>MNPAAEAEFNILLATDSYKVTHYKQYPPNTSKVYSYFECREKKTENSKLRKVKYEETVFYGLQYILNKYLKGKVVTKEKIQEAKDVYKEHFQDDVFNEKGWNYILEKYDGHLPIEIKAVPEGFVIPRGNVLFTVENTDPECYWLTNWIETILVQSWYPITVATNSREQKKILAKYLLETSGNLDGLEYKLHDFGYRGVSSQETAGIGASAHLVNFKGTDTVAGLALIKKYYGTKDPVPGYSVPAAEHSTITAWGKDHEKDAFEHIVTQFSSVPVSVVSDSYDIYNACEKIWGEDLRHLIVSRSTQAPLIIRPDSGNPLDTVLKVLEILGKKFPVTENSKGYKLLPPYLRVIQG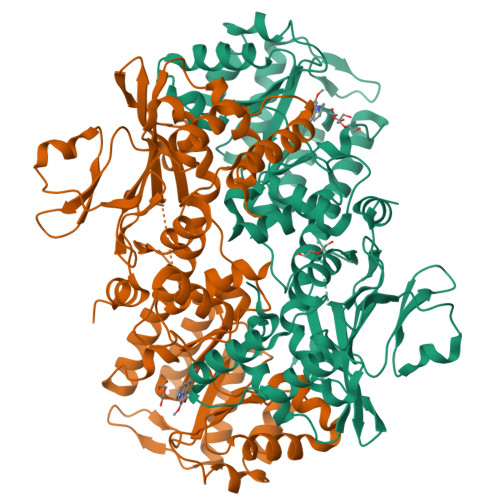DGVDINTLQEIVEGMKQKMWSIENIAFGSGGGLLQKLTRDLLNCSFKCSYVVTNGLGINVFKDPVADPNKRSKKGRLSLHRTPAGNFVTLEEGKGDLEEYGQDLLHTVFKNGKVTKSYSFDEIRKNAQLNIELEAAHH[2x]3-bromo-N-[3-(1H-tetrazol-5-yl)phenyl]-1H-indole-5-carboxamide 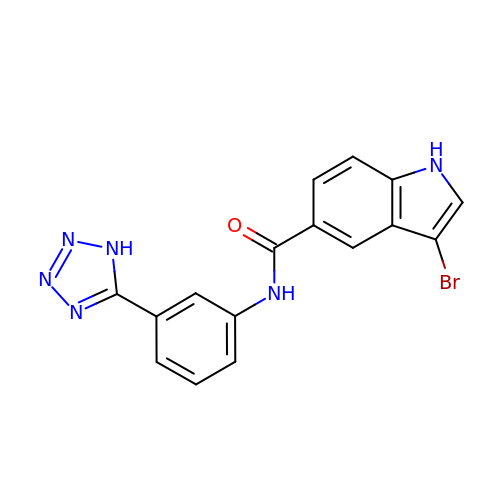| C16 H11 Br N6 O | XFHGTCMLEBYPMZ-UHFFFAOYSA-N Titin has a molecular weight of more than 3 MDa in its longest isoform and is over 1.5 μm in length, spanning half of a sarcomeric unit from the peripheral Z-disk to the central M-band[3–5]. Taking titin kinase as the N-terminal boundary of the titin M-band segment, there are another ten Ig domains towards the far C-terminus of titin, referred to as M1 to M10, encoded by at least six exons 358–363, or Mex1 to Mex6, on the respective TTN gene. To achieve this goal, we have solved the crystal structures of five titin M-band domains: M1, M3, M4, M7, and M10. In addition to the ABDE/A’CC’FG β-sheet sandwich core, all M-band domain structures comprise two characteristic tip regions, which we refer to as “N-tip” and “C-tip” due to their proximity to the N-termini and C-termini of the respective domains.

The structure of the M4 domain was determined in two different crystal forms, with one showing a trimeric M4 domain assembly and the other revealing a disulfide-mediated dimeric state. Two other M-band domains each contain a single exposed cysteine: C20 in the M4 domain (E19 in M1) located at the A’B loop at the C-tip, and C42 in the M10 domain (F42 in M1) located at the tip of the CC’ loop near the C-tip. In one of the two crystal structures of the M4 domain, we found evidence for an intermolecular disulfide bridge across a crystallographic two-fold axis. It is mediated by two exposed cysteines, both C20 from two M4 domains at the C-tip coupled with an intermolecular Zn2+-binding site with tetragonal association of D68 (D68 in M1) and H70 (T70 in M1) from the two interacting M4 domains. By contrast, for domain M4, we found an additional higher molecular peak when using size exclusion chromatography, indicating limited dimerization. Interestingly in the presence of Zn2+, which is found in the structure of the disulfide bridge-mediated M4 tandem arrangement, we detected a further increased level of M4 domain oligomerization. In correlation with our size exclusion data, SDS-PAGE analysis under reducing and non-reducing conditions revealed a covalent higher molecular weight species, indicating intermolecular disulfide bridge formation. We show that two M-band domains with exposed cysteines (M3, M4) have limited potential for disulfide bridge-mediated linkage as purified proteins, additionally supported by a structure of a disulfide bridge-mediated M4 domain dimer (M4-SS-M4’).

> GPFTLDHAPRITLRMRSHRVPCGQNTRFILNVQSKPTAEVKWYHNGVELQESSKIHYTNTSGVLTLEILDCHTDDSGTYRAVCTNYKGEASDYATLDVTGGDY> MSDSVILRSIKKFGEENDGFESDKSYNNDKKSRLQDEKKGDGVRVGFFQLFRFSSSTDIWLMFVGSLCAFLHGIAQPGVLLIFGTMTDVFIDYDVELQELQIPGKACVNNTIVWTNSSLNQNMTNGTRCGLLNIESEMIKFASYYAGIAVAVLITGYIQICFWV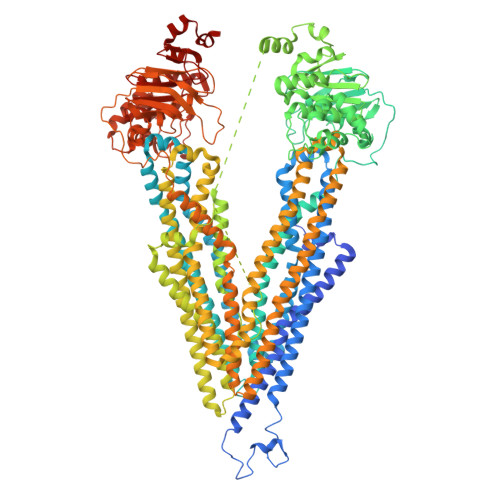IAAARQIQKMRKFYFRRIMRMEIGWFDCNSVGELNTRFSDDINKINDAIADQMALFIQRMTSTICGFLLGFFRGWKLTLVIISVSPLIGIGAATIGLSVSKFTDYELKAYAKAGVVADEVISSMRTVAAFGGGKREVERYEKNLVFAQRWGIRKGIVMGFFTGFVWCLIFLCYALAFWYGSTLVLDEGEYTPGTLVQIFLSVIVGALNLGNASPCLEAFATGRAAATSIFETIDRKPIIDCMSEDGYKLDRIKGEIEFHNVTFHYPSRPEVKILNDLNMVIKPGEMTALVGPSGAGKSTALQLIQRFYDPCEGMVTVDGHDIRSLNIQWLRDQIGIVEQEPVLFSTTIAENIRYGREDATMEDIVQAAKEANAYNFIMDLPQQFDTLVGEGGGQMSGGQKQRVAIARALIRNPKILLLDMATSALDNESEAMVQEVLSKIQHGHTIISVAHRLSTVRAADTIIGFEHGTAVERGTHEELLERKGVYFTLVTLQSQGNQALNEEDIKDATEDDMLARTFSRGSYQDSLRASIRQRSKSQLSYLVHEPPLAVVDHKSTYEEDRKDKDIPVQEEVEPAPVRRILKFSAPEWPYMLVGSVGAAVNGTVTPLYAFLFSQILGTFSIPDKEEQRSQINGVCLLFVAMGCVSLFTQFLQGYAFAKSGELLTKRLRKFGFRAMLGQDIAWFDDLRNSPGALTTRLATDASQVQGAAGSQIGMIVNSFTNVTVAMIIAFSFSWKLSLVILCFFPFLALSGATQTRMLTGFASRDKQALEMVGQITNEALSNIRTVAGIGKERRFIEALETELEKPFKTAIQKANIYGFCFAFAQCIMFIANSASYRYGGYLISNEGLHFSYVFRVISAVVLSATALGRAFSYTPSYAKAKISAARFFQLLDRQPPISVYNTAGEKWDNFQGKIDFVDCKFTYPSRPDSQVLNGLSVSISPGQTLAFVGSSGCGKSTSIQLLERFYDPDQGKVMIDGHDSKKVNVQFLRSNIGIVSQEPVLFACSIMDNIKYGDNTKEIPMERVIAAAKQAQLHDFVMSLPEKYETNVGSQGSQLSRGEKQRIAIARAIVRDPKILLLDEATSALDTESEKTVQVALDKAREGRTCIVIAHRLSTIQNADIIAVMAQGVVIEKGTHEELMAQKGAYYKLVTTGSPIS> MQPGSSRCEEETPSLLWGLDPVFLAFAKLYIRDILDMKESRQVPGVFLYNGHPIKQVDVLGTVIGVRERDAFYSYGVDDSTGVINCICWKKLNTESVSAAPSAARELSLTSQLKKLQETIEQKTKIEIGDTIRVRGSIRTYREEREIHATTYYKVDDPVWNIQIARMLELPTIYRKVYDQPFHSSALEKEEALSNPGALDLPSLTSLLSEKAKEFLMENRVQSFYQQELEMVESLLSLANQPVIHSASSDQVNFKKDTTSKAIHSIFKNA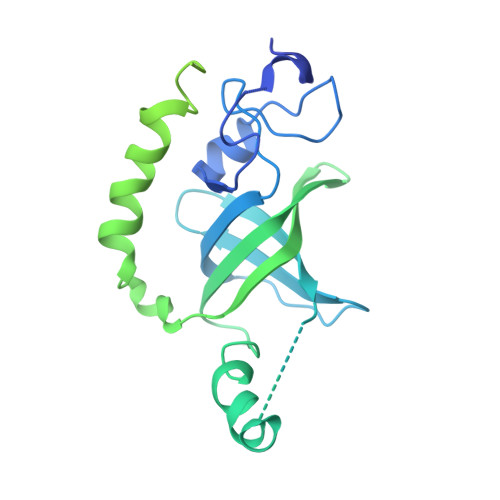IQLLQEKGLVFQKDDGFDNLYYVTREDKDLHRKIHRIIQQDCQKPNHMEKGCHFLHILACARLSIRPGLSEAVLQQVLELLEDQSDIVSTMEHYYTAF> MARQNLKSTDRAVQQMLDKAKREGIQTVWDRYEAMKPQCGFGETGLCCRHCLQGPCRINPFGDEPKVGICGATAEVIVARGLDRSIAAGAAGHSGHAKHLAHTLKKAVQGKAASYMIKDRTKLHSIAKRLGIPTEGQKDEDIALEVAKAALADFHEKDTPVLWVTTVLPPSRVKVLSAHGLIPAGIDHEIAEIMHRTSMGCDADAQNLLLGGLRCSLADLAGCYMGTDLADILFGTPAPVVTESNLGVLKADAVNVAVHGHNPVLSDIIVSVSKEMENEARAAGATGINVVGICCTGNEVLMRHGIPACTHSVSQEMAMITGALDAMILDYQCIQPSVATIAECTGTTVITTMEMSKITGATHVNFAEEAAVENAKQILRLAIDTFKRRKGKPVEIPNIKTKVVAGFSTEAIINALSKLNANDPLKPLIDNVVNGNIRGVCLFAGCNNVKVPQDQNFTTIARKLLKQNVLVVATGCGAGALMRHGFMDPANVDELCGDGLKAVLTAIGEANGLGGPLPPVLHMGSCVD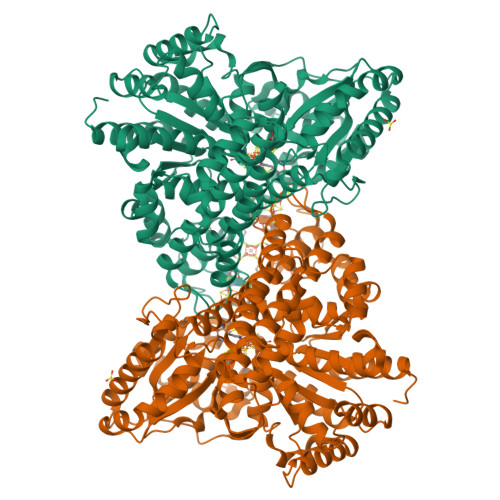NSRAVALVAALANRLGVDLDRLPVVASAAEAMHEHAVAIGTWAVTIGLPTHIGVLPPITGSLPVTQILTSSVKDITGGYFIVELDPETAADKLLAAINERRAGLGLPW> FPPQWICCDIRYLDVSILGKFAVVMADPPWDIHMELPYGTLTDDEMRRLNIPVLQDDGFLFLWVTGRAMELGRECLNLWGYERVDEIIWVKTNQLQRIIRTGRTGHWLNH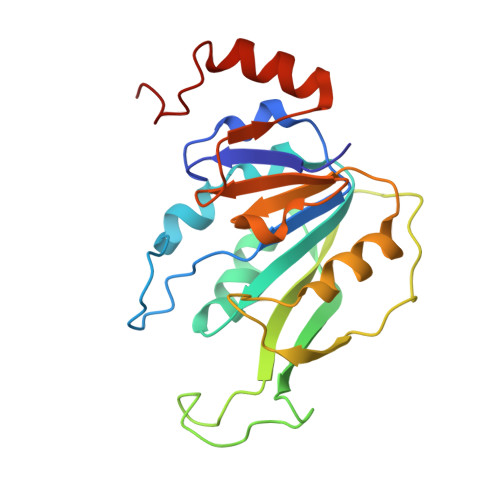GKEHCLVGVKGNPQGFNQGLDCDVIVAEVRSTSHKPDEIYGMIERLSPGTRKIELFGRPHNVQPNWITLGNQLDGIHLLDPDVVARFKQRYPDGIISKPKNL> QLPI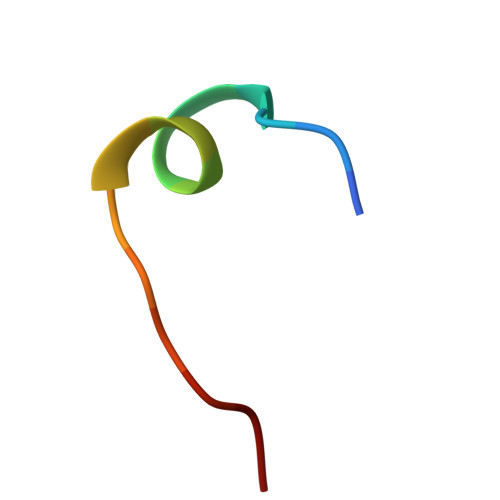LHHAYLPSIGG> TLEPEGAPYWTNTEKMEKRLHA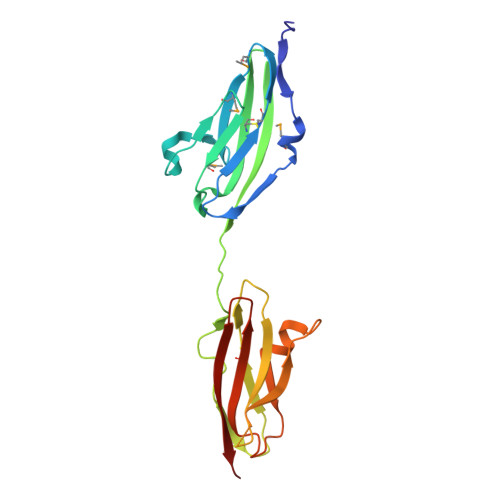VPAANTVKFRCPAGGNPMPTMRWLKNGKEFKQEHRIGGYKVRNQHWSLIMESVVPSDKGNYTCVVENEYGSINHTYHLDVVERSPHRPILQAGLPANASTVVGGDVEFVCKVYSDAQPHIQWIKHVEKNGSKYGPDGLPYLKVLKAAGVNTTDKEIEVLYIRNVTFEDAGEYTCLAGNSIGISFHSAWLTVLPA>[3x]MNMISRRKNAKALSGAVTALILVIASVIIALVVVGFAFGLFGAFTGQGTVTQVGTATLSAGTGTLTVTLKNTGAATQVTGAIINGNAASVSGQVTISAGQNTYSISL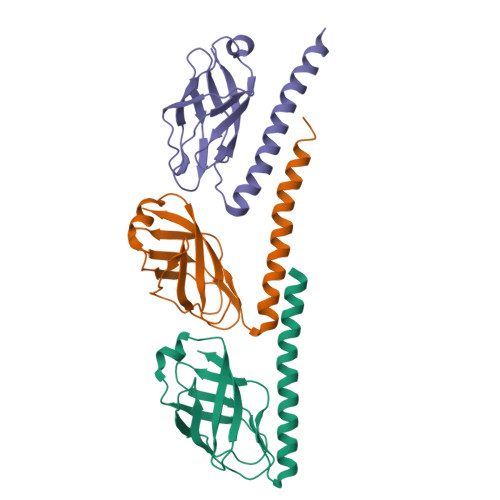GGISSSTLQNLVGSTISLTLQLSNGQTVTVSAIITS pyrrolidine-1-carbaldehyde 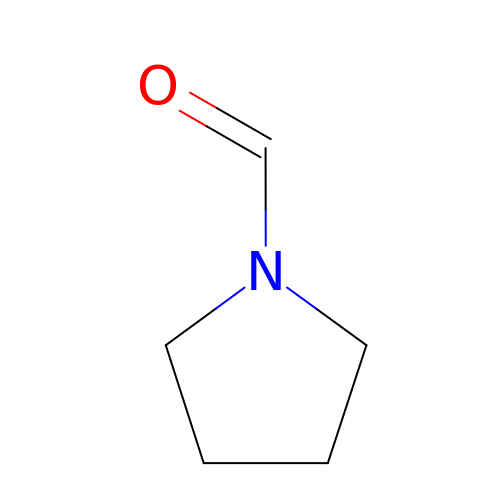| C5 H9 N O | AGRIQBHIKABLPJ-UHFFFAOYSA-N>[2x]MPNRFVIADPKRCLGCYTCIAACAFVHEEQGLQPFPRLYLTYTSEGIMPIQCRHCEDAPCAEVCPVEAIKKEGNAIIIDEKACIGCKTCLLACSFGAIDFSVQDSLEQSIFKDIKENLMQDQKTQQRIVAVKCDLCNFREEGPACVQFCPTKALKLVDGDEINKMVKNKRTVNVESLLSVYGTK;>[6x]MYQKVNCYSILFLKGVDKMKTQLNPFVVANPAKCIGCKACEVACFAVHNRNNHVGATVGTVSIPVIPRLHLIKTEHGTMPIQCRHCEDAPCANVCTVGAIKREGNAIVVDEKLCIGCKSCLLACPFGAIELLPQYEDGREVFQINLKEESESGLVQEPRIIAYKCDLCNDLGEPACVKACPENALTLVMPTEMKKARNKEAALSFLRVVR;>MSANKAIINIDQELCTGCRRCAEVCPVDAIEGEKGKPQKINTEVCVMCGQCVQKCSSYASYFDESITPRNVKLQERGMLDSVKEPLFAAYNLGYARQVKEALENPQLFKVVQCAPAIRVSIAEEFGLDLGDLTPGKLVAALRRLNFDRVYDTNFGADLTIIEEANELVKRIKEGKDLPMFTSCCPAWVKFAEQTYPELLKHISTCKSPQQMTGAIIKTYGAKINNVDPAKIFSVSVMPCTCKSYESDRPEMRSSGYKDVDLVITTRELAHLMKDKGIDFATLPDEEFDSPLGNYTGAATIFGNTGGVMEAALRTAYELITKKPIPNIDIEFVRGGEGIRTATVQVGELELKIAVVSGLKNVIPILEDIKKNKCDLHFVEVMTCPEGCISGGGQPKLLLEEYREVAYKKRKEALYKHDAELELRKSHENPAIKKLYEEFLGEPLGKQSHHLLHTKYT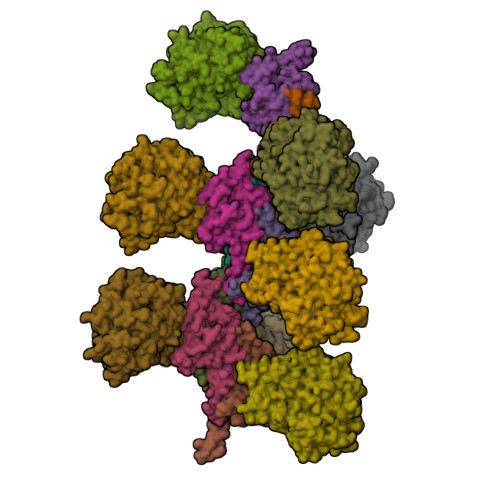PRKKV[6x];>[2x]MKDGKQEKVLTTCPYCGTGCGLYLKVENEKIVGVEPDKLHPVNQGELCIKGYYGYKYVHDPRRLTSPLIKKNGKFVPVSWDEALNFIANGLKKIKSEYGSDAFAMFCSARATNEDNYAAQKFARAVIGINNVDHCARLCHAPTVAGLAMTLGSGAMTNSIPEISTYSDVIFIIGSNTAECHPLIAAHVIKAKERGAKLIVADPRMNAMVHKADIWLRVPSGYNIPLINGMIHIIIKEGLVKTDFVKNHAVGFEEMAKAVEKYTPEYVEELTGIPKKDLIKAARFYGQAQAAAILYSMGVTQFSHGTGNVVSLANLAVITGNLGRPGAGICPLRGQNNVQGACDVGALPNVLPGYLDVTKEQNRERFEKVWGVKLPSNIGLRVTEVPDAILNKRVRALYIFGENPIMSDPDSDHLRHALEHLDLLIVQDIFLTETARLAHVVLPAACWAEKDGTFTNTERRVQRVRKAVEAPGEAKPDWWIFSQIAERMGYTGMQYNNVQEIWDEVRKIVPEKFGGISYARLEKEKGLAWPCPTEDHTGTPILYLGGKFATPSGKAQMYPVIFYPNTCICDEGAEKQDFNHVIVGSIAELPDEEYPFTLTTGRRVYHYHTATMTRKSPVIDQIAPQELVEINPQDATRLGINDGDFLRVSTRRGYVATRAWVTERVPKGTIFMTFHYWEACCNELTNTASDAICCIPEFKVAAAKVEKISQVEAQAILKEKIEKYQVELEKDVANMLAKEKGGK4-(4-methylpiperazin-1-yl)benzonitrile | C12 H15 N3 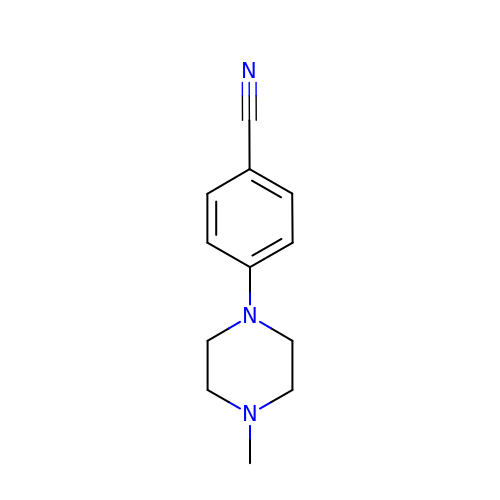| ZSDPKKGOSKXEHN-UHFFFAOYSA-N> MSNFVNLDIFSNYQKYIDNEQEVRENIRIVVREIEHLSKEAQIKLQIIHSDLSQISAACGLARKQVELCAQKYQKLAELVPAGQYYRYSDHWTFITQRLIFIIALVIYLE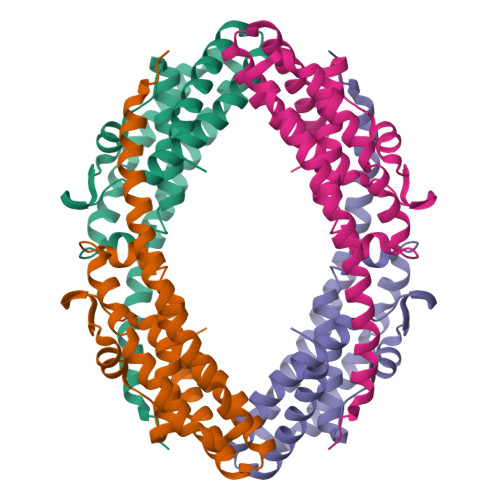AGFLVTRETVAEMLGLKISQSEGFHLDVEDYLLGILQLASELSRFATNSVTMGDYERSLNISHFIGDLNTGFRLLNLKNDGLRKRFDALKYDVKKIEEVVYDVSIRGLSSKEKDQQEEPAVPATE>MKHSLPDLPYDYGALEPHINAQIMQLHHSKHHAAYVNNLNVTEEKYQEALAKGDVTAQIALQPALKFNGGGHINHSIFWTNLSPNGGGEPKGELLEAIKRDFGSFDKFKEKLTAASVGVQGSGWGWLGFNKERG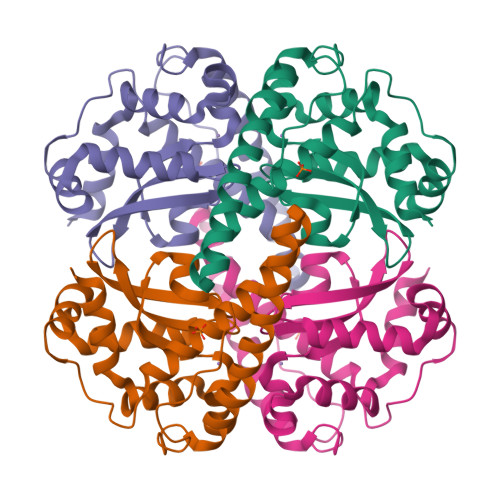HLQIAACPNQDPLQGTTGLIPLLGIDVWEHAYYLQYKNVRPDYLKAIWNVINWENVTERYMACKK[2x]>MFSAGHKIKGTVVLMPKNELEVNPDGSAVDNLNAFLGRSVSLQLISATKADAHGKGKVGKDTFLEGINTSLPTLGAGESAFNIHFEWDGSMGIPGAFYIKNYMQVEFFLKSLTLEAISNQGTIRFVCNSWVYNTKLYKSVRIFFANHTYVPSETPAPLVEYREEELKSLRGNGTGERKEYDRIYDYDVYNDLGNPDKSEKLARPVLGGSSTFPYPRRGRTGRGPTVTDPNTEKQGEVFYVPRDENLGHLKSKDALEIGTKSLSQIVQPAFESAFDLKSTPIEFHSFQDVHDLYEGGIKLPRDVISTIIPLPVIKELYRTDGQHILKFPQPHVVQVSQSAWMTDEEFAREMIAGVNPCVIRGLEEFPPKSNLDPAIYGDQSSKITADSLDLDGYTMDEALGSRRLFMLDYHDIFMPYVRQINQLNSAKTYATRTILFLREDGTLKPVAIELSLPHSAGDLSAAVSQVVLPAKEGVESTIWLLAKAYVIVNDSCYHQLMSHWLNTHAAMEPFVIATHRHLSVLHPIYKLLTPHYRNNMNINALARQSAINANGIIETTFLPSKYSVEMSSAVYKNWVFTDQALPADLIKRGVAIKDPSTPHGVRLLIEDYPYAADGLEIWAAIKTWVQEYVPLYYARDDDVKNDSELQHWWKEAVEKGHGDLKDKPWWPKLQTLEDLVEVCLIIIWIASALHAAVNFGQYPYGGLIMNRPTASRRLLPEKGTPEYEEMINNHEKAYLRTITSKLPTLISLSVIEIASTHASDEVYLGQRDNPHWTSDSKALQAFQKFGNKLKEIEEKLVR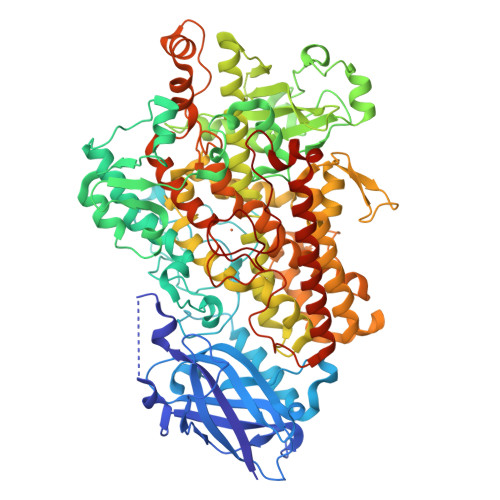RNNDPSLQGNRLGPVQLPYTLLYPSSEEGLTFRGIPNSISI[2x]> SGRFDQYPTKKGDFAIDGYLLDYSSPKQGCWVDGITVYGDIYIGKQNWGTY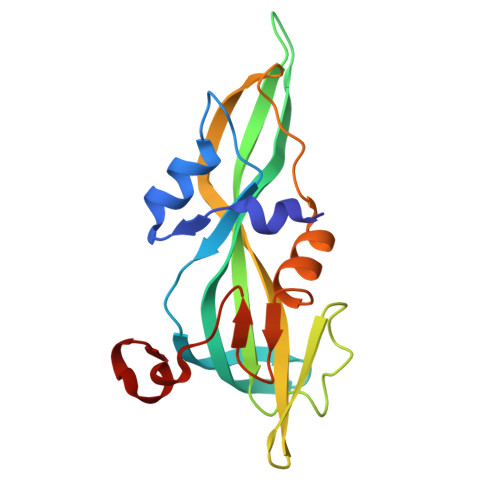TRPVFAYLQYVETISGSGTFVIYQVVLVYAHNATSAGRQNANAFAYSKTQAVGSRVDLYYLSAITQRKRVIVPSSNAVTPLDWDTVQRNVLMENYNPGSNSGHFSFDWSAYNDPHRRY>[3x]GMIYPYKGKTPQIAASAFIADYVTITGDVVIGEETSIWFNTVIRGDVAPTVIGNRVNIQDNSILHQSPNNPLIIEDGVTVGHQVILHSAIVRKNALIGMGSIILDRAEIGEGAFIGAGSL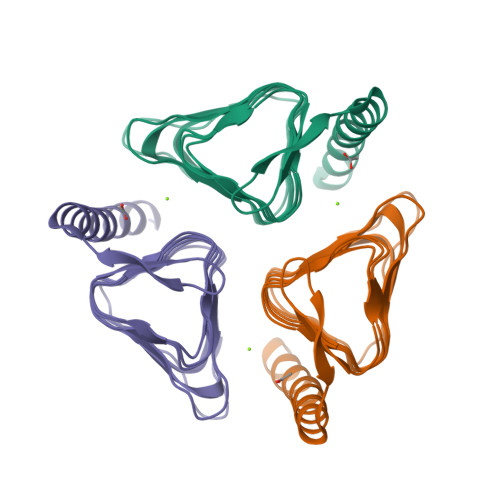VPPGKKIPPNTLALGRPAKVVRELTEDDIREMERIRREYVEKGQYYKALQQQRTSCADKKELP>MNTKYNKEFLLYLAGFVDGDGSIIAQIKPNQSCKFKHQLSLTFQV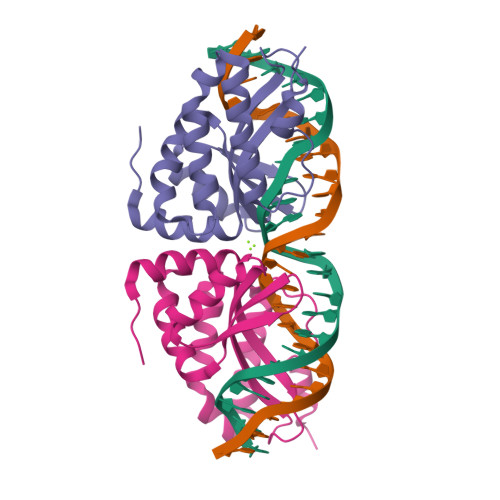TEKTQRRWFLDKLVDEIGVGYVRDRGSVSDYILSEIKPLHNFLTQLQPFLKLKQKQANLVLKIIEQLPSAKESPDKFLEVCTWVDQIAALNDSKTRKTTSETVRAVLDSLSEKKKSSP[2x]>[4x]SMMELRVGNRYRLGRKIGSGSFGDIYLGTDIAAGEEVAIKLECVKTKHPQLHIESKIYKMMQGGVGIPTIRWCGAEGDYNVMVMELLGPSLEDLFNFCSRKFSLKTVL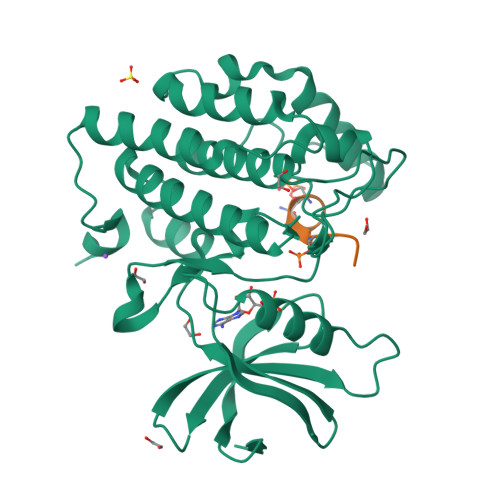LLADQMISRIEYIHSKNFIHRDVKPDNFLMGLGKKGNLVYIIDFGLAKKYRDARTHQHIPYRENKNLTGTARYASINTHLGIEQSRRDDLESLGYVLMYFNLGSLPWQGLKAATKRQKYERISEKKMSTPIEVLCKGYPSEFATYLNFCRSLRFDDKPDYSYLRQLFRNLFHRQGFSYDYVFDWNMLK;>[4x]SSASTVSVGSSY> SNAPRAAGHSEEVLEREASFSLTTIDGEVISLNNVGGDVVILWFMAAWCPSCVYMADLLDRLTEKYREISVIAIDFWTAEALKALGLNKPGYPPPDTPEMFRKFIANYGDPSWIMVMDDGSLVEKFNVRSIDYIVIMDKSSNVLYAGTTPSLGELE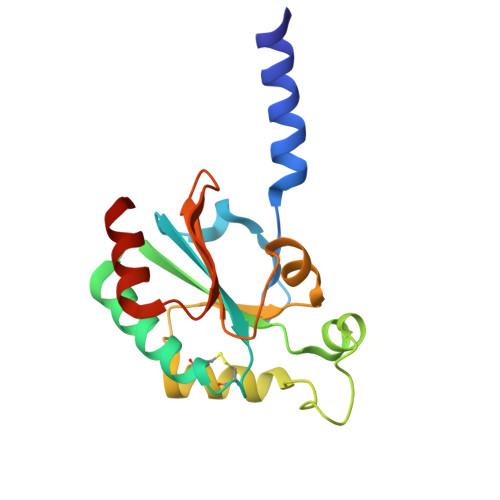SVIKSVQGG> SGAVTSFLHSLIIQNEPRFAMFGPGLEELNTSLVLSLMSSEELCPTAGLPQRQIDGIGSGVNFQLNNQHKFNILILYSTTRKERDRAREEHTSAVNKMFSRHNEGDDQQGSRYSVIPQIQKVCEVVDGFIYVANAEAHKRHEWQDEFSHIMAMTDPAFGSSGRPLLVLSCISQ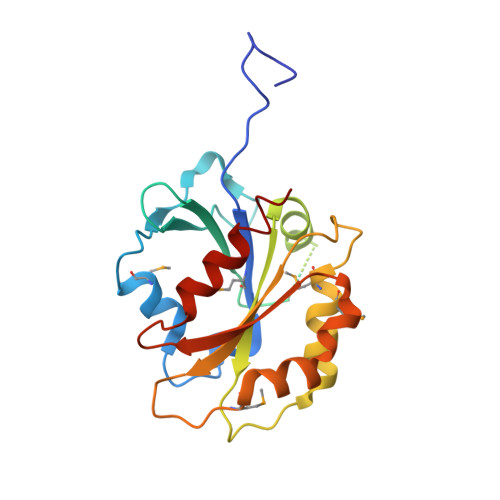GDVKRMPCFYLAHELHLNLLNHPWLVQDTEAETLTGFLNGIEWILEEVESKRAR>[4x]MPLNRTLEMSELPGLEDWEDEFDLENAVLFEVAWEVANKVGGIYTVLQTKAKVTGDEWGDNYFLVGPYTEQGVRTQVELLEAPTPALKRTLDSMNSKGCKVYFGRWLIEGGPLVVLLDVGASAWALERWKGELWDTCNIGVPWYDREANDAVLFGFLTTWFLGEFLAQSEEKPHVVAHFHEWLAGVGLCLCRARRLPVATIFTTHATLLGRYLCAGAVDFYNNLENFNVDKEAGERQIYHRYCMERAAAHCAHVFTTVSQITAIEAQHLLKRKPDIVTPNGLNVKKFSAMHEFQNLHAQSKARIQEFVRGHFYGHLDFNLDKTLYFFIAGRYEFSNKGA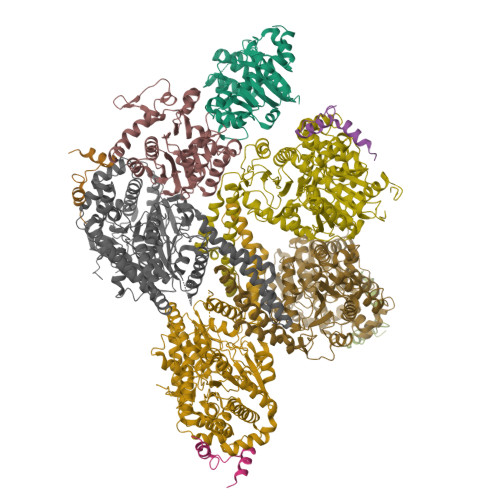DVFLEALARLNYLLRVNGSEQTVVAFFIMPARTNNFNVETLKGQAVRKQLWDTANTVKEKFGRKLYESLLVGSLPDMNKMLDKEDFTMMKRAIFATQRQSFPPVCTHNMLDDSSDPILTTIRRIGLFNSSADRVKVIFHPEFLSSTSPLLPVDYEEFVRGCHLGVFPSYYEPWGYTPAECTVMGIPSISTNLSGFGCFMEEHIADPSAYGIYILDRRFRSLDDSCSQLTSFLYSFCQQSRRQRIIQRNRTERLSDLLDWKYLGRYYMSARHMALSKAFPEHFTYEPNEADAAQGY;>GPMTDQAFVTLTTNDAYAKGALVLGSSLKQHRTTRRLVVLATPQVSDSMRKVLETVFDEVIMVDVLDSGDSAHLTLMKRPELGVTLTKLHCWSLTQYSKCVFMDADTLVLANIDDLFDREELSAAPDPGWPDCFNSGVFVYQPSVETYNQLLHLASEQGSFDGGDQGILNTFFSSWATTDIRKHLPFIYNLSSISIFSYLPAFKVFGASAKVVHFLGRVKPWNYTYDPKTKSVKSEAHDPNMTHPEFLILWWNIFTTNVLPLLQQFGLVKDTCSYVNVLSDLVYTLAFSCGFCRKEDVSGAISHLSLGEIPAMAQPFVSSEERKERWEQGQADYMGADSFDNIKRKLDTYLQ[6x]>[3x]MLSPKAATLAERSAGLAFSLYQAMAKDQAVENILLSPVVVASSLGLVSLGGKATTASQAKAVLSAEQLRDEEVHAGLGELLRSLSNSTARNVTWKLGSRLYGPSSVSFAEDFVRSSKQHYNCEHSKINFRDKRSALQSINEWAAQTTDGKLPEVTKDVERTDGALLVNAMFFKPHWDEKFHHKMVDNRGFMVTRSYTVGVTMMHRTGLYNYYDDEKEKLQIVEMPLAHKLSSLIILMPHHVEPLERLEKLLTKEQLKIWMGKMQKKAVAISLPKGVVEVTHDLQKHLAGLGLTEAIDKNKADLSRMSGKKDLYLASVFHATAFEWDTEGNPFDQDIYGREELRSPKLFYADHPFIFLVRDTQSGSLLFIGRLVRPKGDKMRDELLEHHHHHH;> MLSPKAATLAERSAGLAFSLYQAMAKDQAVENILLSPVVVASSLGLVS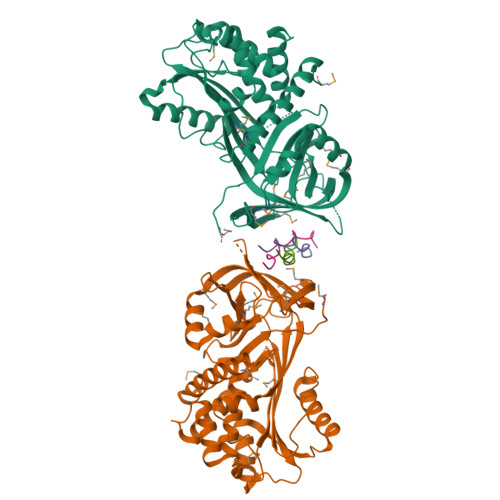LGGKATTASQAKAVLSAEQLRDEEVHAGLGELLRSLSNSTARNVTWKLGSRLYGPSSVSFAEDFVRSSKQHYNCEHSKINFRDKRSALQSINEWAAQTTDGKLPEVTKDVERTDGALLVNAMFFKPHWDEKFHHKMVDNRGFMVTRSYTVGVTMMHRTGLYNYYDDEKEKLQIVEMPLAHKLSSLIILMPHHVEPLERLEKLLTKEQLKIWMGKMQKKAVAISLPKGVVEVTHDLQKHLAGLGLTEAIDKNKSDLSRMSGKKDLYLASVFHATAFEWDTEGNPFDQDIYGREELRSPKLFYADHPFIFLVRDTQSGSLLFIGRLVRPKGDKMRDELLEHHHHHH;>[6x]XPPGPPGPPGPRGPPGPPGX> PPGTVDKKMVEKCWKLMDKVVRLCQNPKLALKNSPPY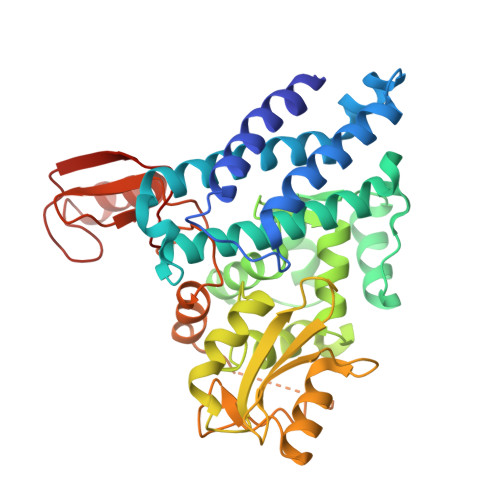ILDLLPDTYQHLRTILSRYEGKMETLGENEYFRVFMENLMKKTKQTISLFKEGKERMYEENSQPRRNLTKLSLIFSHMLAELKGIFPSGLFQGDTFRITKADAAEFWRKAFGEKTIVPWKSFRQALHEVHPISSGLEAMALKSTIDLTCNDYISVFEFDIFTRLFQPWSSLLRNWNSLAVTHPGYMAFLTYDEVKARLQKFIHKPGSYIFRLSCTRLGQWAIGYVTADGNILQTIPHNKPLFQALIDGFREGFYLFPDGRNQNPDLTGLCEPTPQDHIKVTQEQYELYCEMGSTFQLCKICAENDKDVKIEPCGHLMCTSCLTSWQESEGQGCPFCRCEIKGTEPIVVDPFD>[6x]GSHMFYAVRRGRKTGVFL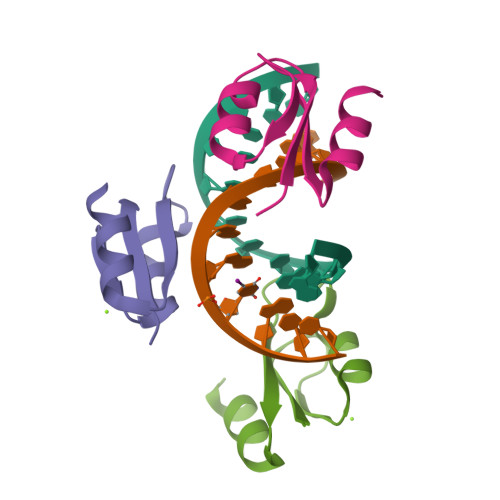TWNECRAQVDRFPAARFKKFATEDEAWAFVRKSAS Stl, the master repressor of the Staphylococcus aureus pathogenicity islands (SaPIs), targets phage-encoded proteins to derepress and synchronize the SaPI and the helper phage life cycles. Our previous work has shown that the Stl repressor, an all-alpha helix protein, is a modular protein composed of an N-terminal domain with the characteristic helix-turn-helix (HTH) folding, which mediates DNA binding, followed by a middle and a C-terminal dimerization domain. Trimeric Duts show high sequence conservation at the residues that make up their active centers, which has been used to define five catalytic motifs (motifs I to V) that are the signature of this family of enzymes. For all these Dut-StlN-ter complexes, the Dut maintains its trimeric state and binds three independent Stl monomers, each of which uses predominantly its middle domain to interact with individual active centers of trimeric Dut.

The hDut-StlN-ter complex was crystallized in the space group P212121, and its asymmetric unit contains one trimer of hDut and three StlN-ter monomers, with a 1:1 assembly identical to both that which was observed in mDut-StlN-ter and that which was previously reported for the ϕ11Dut-StlN-ter complex. In the hDut-StlN-ter complex, the three Stl protomers are well defined with the exception of the 8 to 10 N-terminal residues for which, as in the case of the mDut-StlN-ter complex, no electron density is observable. Surprisingly, in the case of the hDut, the structure allows not only the trace of the main body of each Dut protomer but also the C-terminal motif V. This P-loop, unable to position over the active center occupied by the repressor, is projected toward the Stl and introduces its C-terminal end between the middle domain and the DBD of Stl. The Y116 side chain conformation in the hDut-StlN-ter is identical to that in the ϕ11Dut complex, although its placement is not restricted, because this Dut lacks motif VI. In the hDut-StlN-ter complex, all the Dut C-terminal tails are well ordered, showing a similar mechanism of Stl recognition and complex stabilization by introducing a conserved Phe from Dut motif V in the Stl interdomain hydrophobic pocket. However, C-terminal Dut tail binding is a consequence of the interaction of more than one residue, since the Stl repressor exploits residues from loop α4-α5 (G66, I67, and P68) and the helix α7 (Y98, S99, N102, K103, and N107) to interact with the main and side chains of different Dut motif V residues (D127, R130, G133, G134, and G136). On binding to Stl, the Dut C-terminal tail shows a totally different placement from that observed for nucleotide recognition. In order to allow this drastic change of the C-terminal tail direction, the flexibility provided by several Gly residues and the pivoting interactions of Arg130 at the beginning of the tail are fundamental.

>[3x]YFQGMQLRFARLSEHATAPTRGSARAAGYDLYSAYDYTIPPMEKAVVKTDIQIALPSGCYGRVAPRSGLAAKHFIDVGAGVIDEDYRGNVGVVLFNFGKEKFEVKKGDRIAQLICERIFYPEIEEVQALDDTERGSGGFGSTGKN;>[3x]MEGAGQMAELPTHYGTIIKTLRKYMKLTQSKLSERTGFSQNTISNHENGNRNIGVNEIEIYGKGLGIPSYILHRISDEFKEKGYSPTLNDFGKFDKMYSYVNKAYYNDGDIYYSSYDLYDETIKLLELLKESKINVNDIDYDYVLKLYKQILSTDT>[5x]GSAAAQDMVSPPPPIADEPLTVNTGIYLIESYSLDDCAETFKVNAFLSLSWKDRRLAFDPVRSGVRVKTYEPEAIWIPEIRFVNVENARDADVVDISVSPDGTVQYLERFSARV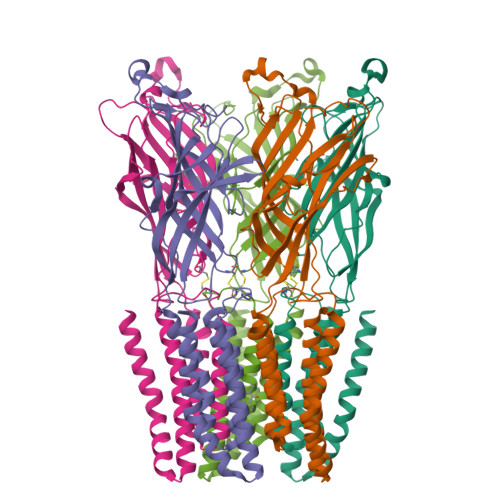LSPLDFRRYPFDSQTLHIYLIVRSVDTRNIVLAVDLEKVGKNDDVFLTGWDIESFTAVVKPANFALEDRLESKLDYQLRISRQYFSYIPNIILPMLFILFISWTAFWSTSYEANVTLVVSTLIAHIAFNILVETNCPKTPYMTYTGAIIFMIYLFYFVAVIEVTVQHYLKVESQPARAASITRASRIAFPVVFLLANIILAFLFFGF>MIVLFVDFDYFYAQVEEVLNPSLKGKPVVVCVFSGRFEDSGAVATANYEARKFGVKAGIPIVEAKKILPNAVYLPMRKEV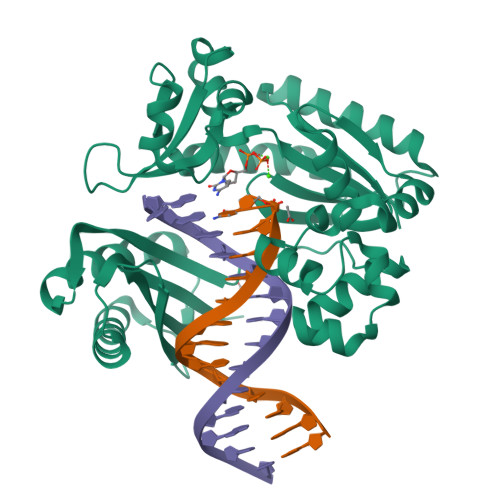YQQVSSRIMNLLREYSEKIEIASIDEAYLDISDKVRDYREAYNLGLEIKNKILEKEKITVTVGISKNKVFAKIAADMAKPNGIKVIDDEEVKRLIRELDIADVPGIGNITAEKLKKLGINKLVDTLSIEFDKLKGMIGEAKAKYLISLARDEYNEPIRTRVRKSIGRIVTMKRNSRNLEEIKPYLFRAIEESYYKLDKRIPKAIHVVAVTEDLDIVSRGRTFPHGISKETAYSESVKLLQKILEEDERKIRRIGVRFSKFIEA[2x]>[8x]MGSDKIHHHHHHMVIGVTGKIGTGKSTVCEILKNKYGAHVVNVDRIGHEVLEEVKEKLVELFGGSVLEDGKVNRKKLAGIVFESRENLKKLELLVHPLMKKRVQEII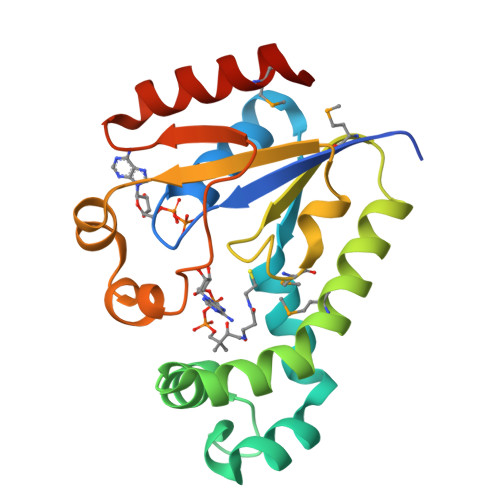NKTSGLIVIEAALLKRMGLDQLCDHVITVVASRETILKRNREADRRLKFQEDIVPQGIVVANNSTLEDLEKKVEEVMKLVWEKRE>[4x]GAMGSPGDGAGASRQRKLEALIRDPRSPINVESLLDGLNSLVLDLDFPALRKNKNIDNFLNRYEKIVKKIRGLQMKAEDYDVVKVIGRGAFGEVQLVRHKASQKVYAMKLLSKFEMIKRSDSAFFWEERDIMAFANSPWVVQLFY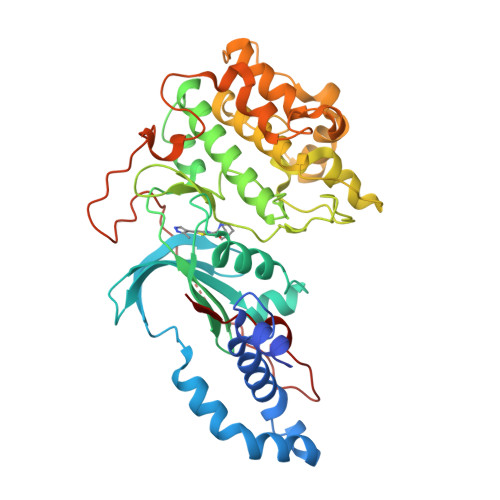AFQDDRYLYMVMEYMPGGDLVNLMSNYDVPEKWAKFYTAEVVLALDAIHSMGLIHRDVKPDNMLLDKHGHLKLADFGTCMKMDETGMVHCDTAVGTPDYISPEVLKSQGGDGYYGRECDWWSVGVFLYEMLVGDTPFYADSLVGTYSKIMDHKNSLCFPEDAEISKHAKNLICAFLTDREVRLGRNGVEEIRQHPFFKNDQWHWDNIRETAAPVVPELSSDIDSSNFDDIEDDKGDVETFPIPKAFVGNQLPFIGFTYYR>VHINKGGRPRQHLLSLTRRAQKHRLRELKIQVKEFADKEEGGDVKAVCLTLFLLALRARNEHRQADELEAIMQGRGSGLQPAVCLAIRVNTFLSCSQYHKMYRTVKAITGRQIFQPLHALRNAEKVLLPGYHPFEWQPPLKNVSSRTDVGIIDGLSGLASSVDEYPVDTIAKRFRYDSALVSALMDMEEDILEGMRSQDLDDYLNGPFTVVVKESCDGMGDVSEKHGSGPAVPEKAVRFSFTVMRITIEHGSQNVKVFEEPKPNSELCCKPLCLMLADESDHETLTAILSPLIAEREAMKSSELTLEMGGIPRTFKFIFRGTGYDEKLVREVEGLEASGSVYICTLCDTTRLEASQNLVFHSITRSHAENLQRYEVWRSNPYHESVEELRDRVKGVSAKPFIETVPSIDALHCDIGNAAEFYKIFQLEIGEVYKHPNASKEERKRWQATLDKHLRKRMNLKPIMRMNGNFARKLMTQETVDAVCELIP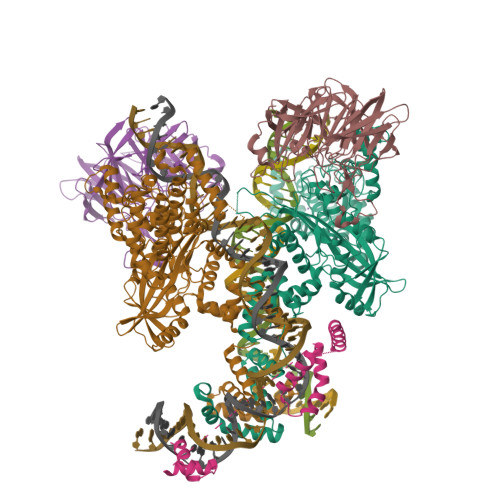SEERHEALRELMDLYLKMKPVWRSSCPAKECPESLCQYSFNSQRFAELLSTKFKYRYEGKITNYFHKTLAHVPEIIERDGSIGAWASEGNQSGNKLFRRFRKMNARQSKCYEMEDVLKHHWLYTSKYLQKFMNAHNA[2x];>MSLQMVTVGHNIALIQPGFSLMNFDGQVFFFGQKGWPKRSCPTGVFHFDIKQNHLKLKPAIFSKDSCYLPPLRYPATCSYKGSIDSDKHQYIIHGGKTPNNELSDKIYIMSVACKNNKKVTFRCTEKDLVGDVPEPRYGHSIDVVYSRGKSMGVLFGGRSYMPSTQRTTEKWNSVADCLPHVFLIDFEFGCATSYILPELQDGLSFHVSIARNDTVYILGGHSLASNIRPANLYRIRVDLPLGTPAVNCTVLPGGISVSSAILTQTNNDEFVIVGGYQLENQKRMVCSLVSLGDNTIEISEMETPDWTSDIKHSKIWFGSNMGNGTIFLGIPGDNKQAMSEAFYFYTLRCSEEDLSEDQ[2x];> MGKGDPKKPRGKMSSYAFFVQTCREEHKKKHPDASVNFSEFSKKCSERWKTMSAKEKGKFEDMAKADKARYEREMKTYIPPKGETKKKFKDPNAPKRPPSAFFLFCSEYRPKIKGEHPGLSIGDVAKKLGEMWNNTAADDKQPYEKKAAKLKEKYEKDIAAYR> MATSSSGVDNEISLDSPMPIFNESSTLKPIRVAGVVTTGTDHIDPSVLQAYLDDTIMKSITLGQLVKNADVLNKRLCQHHIALNAKQSFHFQGNTYISDEKETHDVVPLMEVVSQLDILPPKTFTAKTGTNFGNDNDAEAYLQFEKLIDKKYLKLPTRVNLEILRGTKIHSSFLFNSYSSLSPQSILNLKVFSQFYNWNT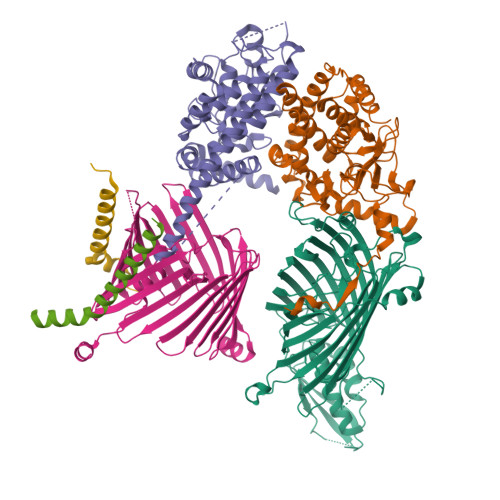NKGLDIGQRGARLSLRYEPLFLHKLLHNPHSNESPTLFHEWFLETCWRSTKICSQGTSAPYMYSGTMLSQAGDQLRTILGHTFVLDKRDHIMCPTKGSMLKWSNELSPGKHLKTQLELNSVKSWMNDDFITFSTTIKTGYLKNLSSQQSLPVHICDKFQSGGPSDIRGFQTFGLGPRDLYDAVGGDAFVSYGLSVFSRLPWKKVEKSNFRLHWFFNGGKLVNHDNTSLGNCIGQLSKEHSTSTGIGLVLRHPMARFELNFTLPITAHENDLIRKGFQFGLGLAFL;> MVSSFSVPMPVKRIFDTFPLQTYAAQTDKDEAVALEIQRRSYTFTERGGGSSELTVEGTYKLGVYNVFLEANTGAALATDPWCLFVQLALCQKNGLVLPTHSQEQTPSHTCNHEMLVLSRLSNPDEALPILVEGYKKRIIRSTVAISEIMRSRILDDAEQLMYYTLLDTVLYDCWITQIIFCASDAQFMELYSCQKLSGSIVTPLDVENSLLQKLSAKSLKISLTKRNKFQFRHREIVKSMQGVYHNHHNSVNQEQVLNVLFENSKQVLLGLKDMLKSDGQPTYLHLKIASYILCITNVKEPIKLKTFVENECKELVQFAQDTLKNFVQ;> MVKGSVHLWGKDGKASLISVDSIALVWFIKLCTSEEAKSMVAGLQIVFSNNTDLSSDGKLPVLILDNGTKVSGYVNIVQFLHKNICTSKYEKGTDYEEDLAIVRKKDRLLEYSLLNYVDVEISRLTDYQLFLNTKNYNEYTKKLFSKLLYFPMWYNTPLQLRSQARENCEEIIGSLTLEDDEEFVESKAMESASQLAQSKTFKIAHKNKIKGKQELQQVKYNLQFDNRLQSCVSNWLAARKKLDDSVILSSDLLFLANLYVQLGLPDGNRIRSKLEQTFGSELLNSMSNKIDDFVHRPSNNLEQRDPQFREQGNVVMSLYNLACKYILEDYKDHDGDYKDHDIDYKDDDDK;> MASAPTPLAEASQIPTIPALSPLTAKQSKGNFFSSNPISSFVVDTYKQLHSHRQSLELVNPGTVENLNKEVSRDVFLSQYFFTGLRADLNKAFSMNPAFQTSHTFSIGSQALPKYAFSALFANDNLFAQGNIDNDLSVSGRLNYGWDKKNISKVNLQISDGQPTMCQLEQDYQASDFSVNVKTLNPSFSEKGEFTGVAVASFLQSVTPQLALGLETLYSRTDGSAPGDAGVSYLTRYVSKKQDWIFSGQLQANGALIASLWRKVAQNVEAGIETTLQAGMVPITDPLMGTPIGIQPTVEGSTTIGAKYEYRQSVYRGTLDSNGKVACFLERKVLPTLSVLFCGEIDHFKNDTKIGCGLQFETAGNQELLMLQQGLDADGNPLQALPQLLESAGKPIPNPLLGLDST;> MAMFGLPQQEVSEEEKRAHQEQTEKTLKQAAYVAAFLWVSPMIWHLVKKQWK;> MADGMFAMPGAAAGAASPQQPKSRFQAFKESPLYTIALNGAFFVAGVAFIQSPLMDMLAPQL1-(4-amino-2-butyl-1H-imidazo[4,5-c]quinolin-1-yl)-2-methylpropan-2-ol | C18 H24 N4 O | 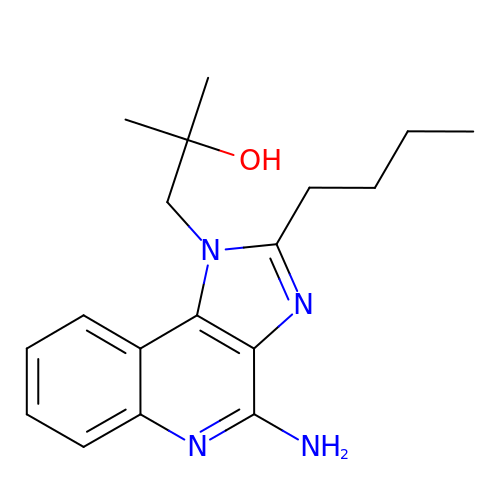GITVQUOQRHRGQQ-UHFFFAOYSA-N>ARPCIPKSFGYSSVVCVCNATYCDSFDPPTFPALGTFSRYESTRSGRRMELSMGPIQANHTGTGLLLTLQPEQKFQKVKGFGGAMTDAAALNILALSPPAQNLLLKSYFSEEGIGYNIIRVPMASCDFSIRTYTYADTPDDFQLHNFSLPEEDTKLKIPLIHRALQLAQRPVSLLASPWTSPTWLKTNGAVNGKG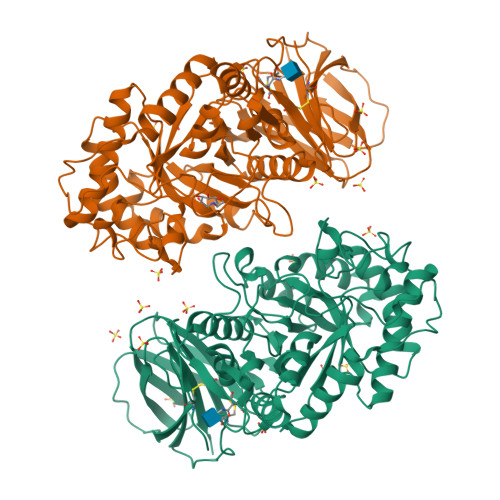SLKGQPGDIYHQTWARYFVKFLDAYAEHKLQFWAVTAENEPSAGLLSGYPFQCLGFTPEHQRDFIARDLGPTLANSTHHNVRLLMLDDQRLLLPHWAKVVLTDPEAAKYVHGIAVHWYLDFLAPAKATLGETHRLFPNTMLFASEACVGSKFWEQSVRLGSWDRGMQYSHSIITNLLYHVVGWTDWNLALNPEGGPNWVRNFVDSPIIVDITKDTFYKQPMFYHLGHFSKFIPEGSQRVGLVASQKNDLDAVALMHPDGSAVVVVLNRSSKDVPLTIKDPAVGFLETISPGYSIHTYLWHRQ[4x]2-[5-AMINO-6-OXO-2-(2-THIENYL)-1,6-DIHYDROPYRIMIDIN-1-YL)-N-[3,3-DIFLUORO -1-ISOPROPYL-2-OXO-3-(N-(2-MORPHOLINO ETHYL)CARBAMOYL]PROPYL]ACETAMIDE | 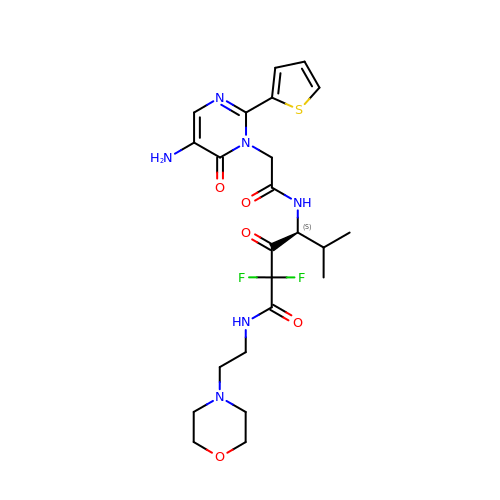C23 H30 F2 N6 O5 S | SZYHELVLDPKTOS-SFHVURJKSA-N> MMLSATQPLSEKLPAHGCRHVAIIMDGNGRWAKKQGKIRAFGHKAGAKSVRRAVSFAANNGIEALTLYAFSSENWNRPAQEVSALMELFVWALDSEVKSLHRHNVRLRIIGDTSRFNSRLQERIRKSEALTAGNTGLTLNIAANYGGRWDIVQGVRQLAEKVQQGNLQPDQIDEEMLNQHVCMHELAPVDLVIRTGGEHRISNFLLWQIAYAE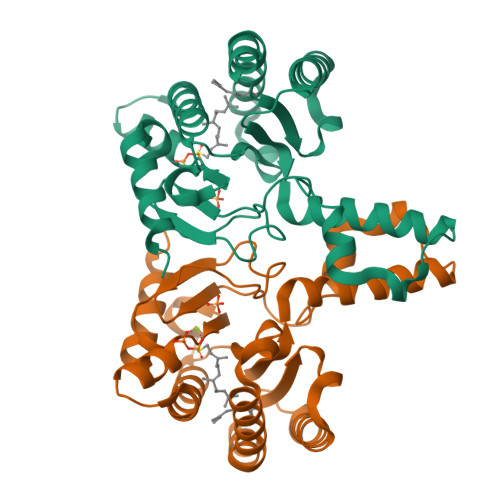LYFTDVLWPDFDEQDFEGALNAFANRERRFGGTEPGDETA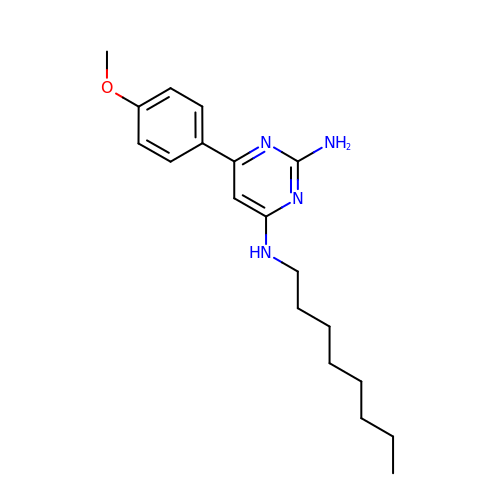6-(4-methoxyphenyl)-N~4~-octylpyrimidine-2,4-diamine | C19 H28 N4 O | HPTZTRACBOHBMX-UHFFFAOYSA-N> MVYVNSVCHMKAAATAGKVEGEGDMQKKFPLAAISKVITTLWAIEKLGVDYRHKTVLHLTPTANGSMDLHVEGSRDPIFGRNLSYFLISELNRMKVTKIENLTFDENFLLDWLAEESPRIGGVTPRYETIE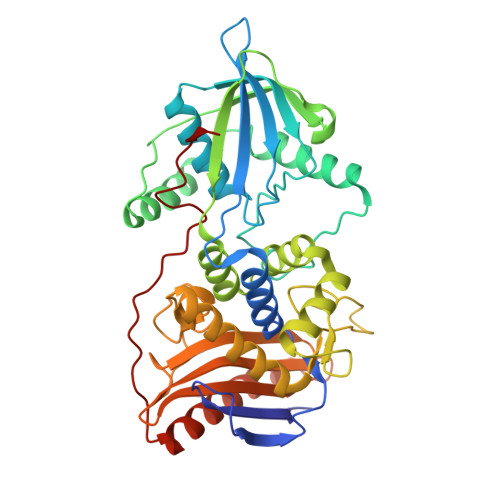QQAEAVIKNLKESFSTAINRAMYSKLRERATKAKVFMLEKPTIEVRNISFLPKNNYKKDKYTGSVVLQSAPLRTILKRMNNQSNNYIADNLYWNLGGTAAFNAFAAATLKADQNQIVFHNGSGNNEGTTAKPIYNEATCETMIKTLYTLNKSLEAKGYKLSDVLSVANKDSDSTIDNFGGNAAGSMIAKTGTVNKAKTLAGSISTKEGEFYFAILLHTDMDQSSSDRGVASQMIKNKISQLINKRSGPKEIQYTEILALPFDQNSYLTEA>SSVLASCPKKPVSSYLRFSKEQLPIFKAQNPDAKTTELIRRIAQRWRELPDSKKKIYQDAYRAEWQVYKEEISRFKEQLTPSQIMSLEKEIMDKHLKRKAMTKKKELTLLGKPKRPRSAYNVYVAERFQEAKGDSPQEKLKTVKENWKNLSDSEKELYIQHAKEDETRYHNEMKSWEEQMIEVGRKDLLRRTIKKQR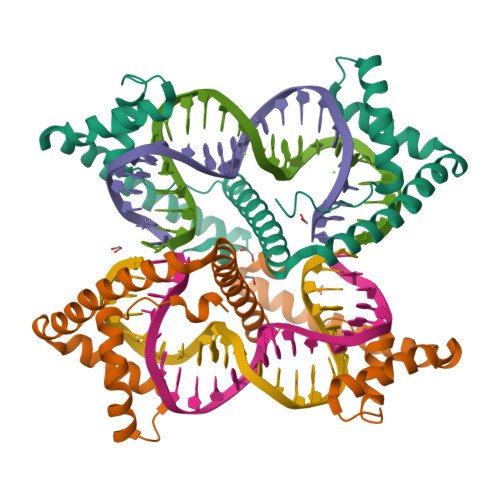KYGAEEC[2x]> AFQVEQYYFDVAEVEAWLGEQELLMMSEDKGKDEQSTLQLLKKHLQL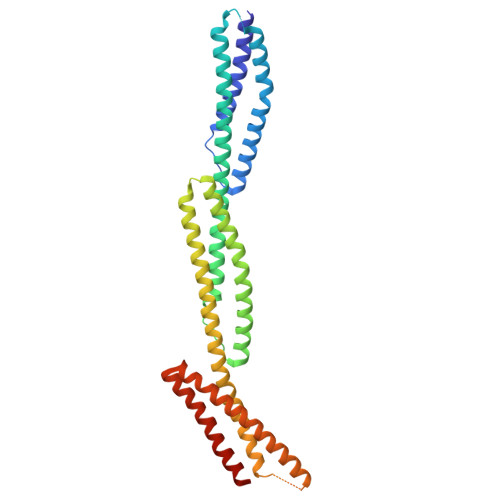EQGVENYEESIAQLSRQCRALLEMGHPDSEQISRRQSQVDRLYVALKELGEERRVSLEQQYWLYQLSRQVDELEHWIAEKEVVAGSPELGQDFEHVSVLQEKFSEFASETGTAGRERLAAVNQMVDELIECGHTAAATMAEWKDGLNEAWAELLELMGTRAQLLAASRELHKFFSDARELQGQIEEKRRRLPRLTAPPEPRPSASSMQRTLRAFEHDLQLLVSQVRQLQEGAAQLRTVYAGEHAEAIASREQEVLQGWKELLAACEDARLHVSST>[2x]APLAPPLAEDRSYRTWRVEDYVEAWERYHGREMTEDERENLARGCIGVTVVNLNREDLSNPPLNLSFGSLRTAEAVQAAL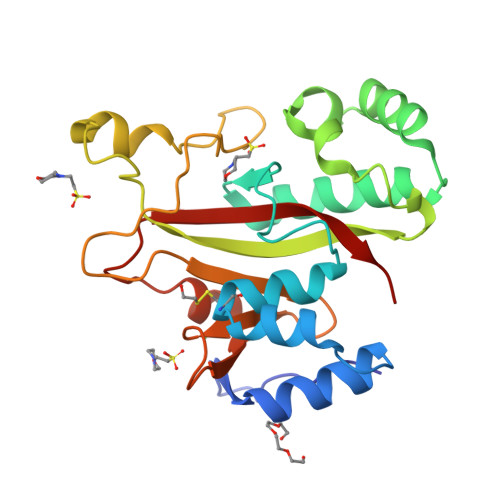NKIVDTHPSPAQYEAAVAKDPILKRLKNVVKALPSWIDSAKLKASIFSKRFYSWQNPDWSEERAHTTYRPDRETDQVDMSTYRYRARPGYVNFDYGWFDQDTNTWWHANHEEPRMVVYQSTLRHYSRPLQDFDEQVFTVAFAKKD> GGLEKDFLPLYFGWFLTKKSSETLRKAGQVFLEELGNHKAFKKELRHFISGDEPKEKLELVSYFGKRPPGVLHCTTKLCDYGKAAGAEEYAQQEVVKRSYGKAFKLSISALFVTPKTAGAQVVLTDQELQLWPSDLDKPSASEGLPPGSRAHVTLGCAADVQPVQTGLDLLDILQQVKGGSQGEAVGELPRGKLYSLGKGRWMLSLTKKMEVKAIFTGYYG

2′,3′-cyclic nucleotide 3′-phosphodiesterase (CNPase) comprises 4% of total myelin protein in the central nervous system (CNS), being the most abundant CNS non-compact myelin protein4. CNPase consists of an N-terminal polynucleotide kinase-like domain10, a catalytic phosphodiesterase domain11, and a membrane-anchored C-terminal tail, which contains a cysteine residue that undergoes isoprenylation. The catalytic domain enables the rapid hydrolysis of nucleoside 2′,3′-cyclic phosphates to nucleoside 2′-phosphates. The CNPase catalytic site, lying in a groove between two lobes, has pseudo two-fold symmetry and contains two apposing His-X-Thr-X (X denotes a hydrophobic residue) motifs, characteristic for 2H phosphoesterases 113537.

While recognizing the caveat that the high KM for these mutants makes kcat rather inaccurate, this implies that the π-π stacking between Phe235 and the nucleotide base is not only required for substrate affinity, but it also may define correct substrate docking into a productive binding mode. In the F235L structure, the flexible active site β5-α7 loop (amino acids 319 – 321) is in the closed conformation. This loop is often found in a mixed conformation, and its conformation depends on the reaction step. As the active site of dCNPcat is empty in the crystal structure, we determined an additional structure of CNPcat with no ligand bound; this was successful when using the F235L mutant. All earlier structures have included either nucleotides or buffer components. The positions of the active-site water molecules, as well as side chain conformations of catalytic residues were nearly identical in dCNPcat and F235L, suggesting any changes in activity of dCNPcat are related to the replacement of H by D in the protein, solvent, and exchangeable sites of the substrate. Our observations allow us to speculate on active-site dynamics that take place during and after catalysis: The β5-α7 loop in both dCNPcat and F235L is closed, confirming the closed state of the active site in the apo form.>MDFQDYIQSLKKDFKLVKINDHTYILHKNKKTLELTPDKMYNIQEINDILNVSYPDISYDRNLEDLGSKNKGILNGFGNVGEDDLHPQIGRRKGKKKGAIFSPEEFKEEEDSDGIDKTDIFPLKKKRDPDSDHFKKTGGDDDNPFLY[2x];>[2x]MFLDTHKQLTLFTSEGKLDQCDNALKAATQGSLSVGCVSENGVVLASLKESNNLVILSEYKKIYQISPNLGITYSGCQPDFRIQYNLSLKISEEYTDIYSTNIPIRLFVEQFSRQIQEYTIKKGYRPFGTLLLIVGDNKMYRVDPSGSYTSLQVGTIGREYTESGRLLERRKGMLDDNISTCVECIREYCGRSVKSEDIDIGVYRGQEFRVYSKEEVQEVFDSINKI;>MSSNTFTEEGRLLQTEYAIKNVSKGGTIIGLVCKDGVILLGINKTELLDEREKIYKINPKVYVSVSGLFGDAMLLKKYGQVKAQDFLYEFDYDCDIDRICNFISEKKQLFTQYNSTRPFGFSFIYAGMKNNKFKLCSTDPSGTINEWKGVCFGENEDAINNGLRNDFPDEEMDMERGLFEIFKILSKVTECSAKDHKKYEILYFKNEESRFLEFEEIENILLRIEEEKNKK[2x];>[2x]MEYENALGIFSPDGRLIQVEYAQQASEQGSLVVFSSDTNEICLSIETKTHNKMLIDQNKLLPVDKDLNIWYTFSGIKPDSYKVLNEARLICRNYKIKTGTNISFDELAYELSLYKQKFTLDSSMRPFGIRSILLQVKDMAKIYVLEPDGNYSEYKCGAVGQKSVSVCEYLEKCEEEDIIFRSVSGLGTVVQSDKNKVMSYVISKDEIRRVEDETVSQIISTVSVK;>[2x]MSIVSRQNANTYSAEGRLYQVEYAMQAMNLGTSSIGIKTKDYVLLASEKKIISKLQNPSSVKKHYRVYDHIALGFSGISADVKTIVDKSRNFAINHEYLYDENCKVERLLEHLADLSLNFDKKEADEKIFSRPFGASLLIIGYDTEPRLFSLDPSGSYLEYHAKAIGSGSEVIENMLEQEFDPNVDINSGLKNILNMLSKVMKDKINNFNVEITAITKNECKILTPEEIEQFLE;>[2x]MNSQTDYTNYIIFNPEGKIKQLEFINNTVQLGSTVVALKNKSFGVFVTYNEKRSKFALQQKKIFPINSKSLFSFSGITNDGTKIVKYLKNSTVFENIRKGRDIHPIHVFDDLCYSACIRTLTNGNRLYGVQGLLLTDYQGISLVLFDPKGSAKEVRGMSIGSRSQSCRTILEDECDKFEEYNKEELVRLGIKALRNAYPETGVLNKDNVDIWILETNQESKQIKSEEYLQ;>MAILDVDTVYTNTGDILQIGYAQKAADNGNTAICMKNKKGLIMIAEKPIESKLYVSEKNFRIKKVNNSIFQISSGIETDLVYINENLKNNLISEKHSNDMDVSHESVRNQIVNIIHQFTRYSGVRPIGINLLTCSKYKNEYKILQTDCTGKSLFFKSSVIGKGSRIVKTELEKLNLENMEIRDLVENGIRILYKSYDPLKDKPFDIEIGIMCEETNGEFVRLEKNQYSEIIEKYKDFSVDGEE[2x];>MSIKDEIYNIFNADGKILQIEYGLEAVNKSLPLVVLKNKNMIVCAAKKNQGHLLEDEVQTSFQPIYPNLYSAFTGNWADVFYVNSKAKDLAHYASYKLGFSVTPDILCRKLADELQPLIQSTGERAPAFAGALFGFDNGKPVVYMTNISAVCYPVYGSMVGSKNQNMYKYVEKYYNEDIEDEKLFEVAVGGLLESLGENSVYQEMEVAYLRNGEVLKYLDDKEIESLLLSIADK[2x];>[2x]MFTKTGTTIVGVKYKGGVVICADTRSTSGPIVADKNCSKIHYISDNIQACGAGTSADITRVTRKASKVLSIFSKTYNRLPRVSHCVRTCQLHLHPYQGHISAALVVGGVDDTGAHLYDVYPHGSSNSVSYTALGSGSLAAISILEAGYKDMNREEAMELACAAIEAGIMNDLYSGSNIDVCVISQEGREMFRNYKKVGVRNEVPKFQYPRSSVKILKEDIYKYIEEK;>[2x]MSDISQHYGGSLLAMIGKSSVAFLSDKRLGSGPISVSKNFTKIYSLTPRLFFGFTGLVSDGEMLFKKIRKNYNLFVQDNNKDMEPSELSNMISYILYQKRLQPYYVAVIVCGMTLDKKPYASSMDCIGAMKETSEFVTSGTASKNLMGLSEALFYPEMEDEDLFTTSVQTFLNSSDRDTFGGMGFECLLINPEGYKRREFVGRCD;>MESSVALKGNDFVIIGTDSSVKNSYLVLKREEDKFYNINNKVVFTYLGDQGDAFRTSSFINEKLVYEEIQNNVEITPKVTANVIQKTLYDNLRSHPKNCYFLVGGLSQDGPELYSVDLYGSLHENDFMAVGISTYFCYGVLDKEYHKNITKEDGIKIIQKCFDVLKQRCSVDISNIEIKIVSKEGVETINKVL[2x];>MEKLFTGDIMEIQNTKVDSAFMKNKIVPYKGTTTLAFIFQGGMVIAVDSRASAGSYIASQNVHKVIRVNKHLIGTMAGGASDCYFWEKKMGLYAKL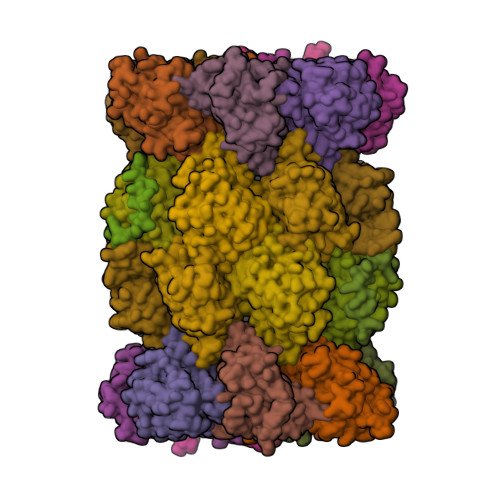YELKNNKRISVSAASMYLSNCVYSYKGQGLSLGSMVCGYDGDKPVIYYVDDAGQRLSGDLFSVGSGSTIAYGVLNESYRFDLTKEEALNLGKKAIWHATHRDAYSGGNVNLYFMDKNGWEHLGTFDVDKFEQ[2x];>MFTLQANTKDQIIKDLNIGDLTIRDLNIKDLNIGDSSTVNLFKVDIPLLSNEIPLDFTFDNLPSNKKEIFESFDSFTDFVEGKTKSQESKFNPYEDNSGSTVSIRLNNSIIIAADTRHCSEMGIYSRNTSKIFRIGDFLLTITGFYADGYELYNRLKYQVQIYESFNKISIHSLANLASKIMYSKRLFPYYSYVTLSGFEGDNPYVYSFDCLGHFEEVDSVCNGSGSPLIQPLLDSTIEKKNWAGENYEVTEEYVKDIVRRGFNAASERDVKTGDNVEIWIIKKDGMTKEYERLRQD[2x];>[2x]MKNFVIGSGVISLRYKNGVITCTDTQASYGNLCKFNDVRRIFRLSSNTLISLSGEISDIQFLMNELNKLNESDPVKMSPRGYLNLVQGILYNKRSRVEPLNVSVSIVGVDDDDFLVSCVNHLGNFYEDNIVCTGLSNMIALPFLRTCNVLDLERDEAISLVEKAMTVMCYRSCRSSNRIQIGVVEKGLVDISDPYVLNTDWQVGHNEEEIVL;>[2x]MVAYDNKNNEGFSPNLPEMTGTTIMAVKYADGILIGADCRTSMGTYVSSRFTDKLTKISDNIYCCRSGSAADTQAITQYITELVQRSSFIDKEIPSVKKAAMAAKDIIYRYPNMLAGLIIAGYDTKPRIFNISLGGTMTEAEWQIGGSGSAYIYGLCDTTFKPNMNLEEALEFVKLAVTCAIKRDNASGGCIRMASITREGVQRFFYSGDKILNST>[2x]RLTSKQTFASFQQWAEKAEALGRDTEIGIYMIYKRDTPDTTPMNAAEQEHYLETLQALDNKKNLIIRPQIHDDREEEELDLGRYIAEDRNARTGFFRMVPKDQRAPETNSGRLTIGVEPKYGAQLALAMATLMDKHKSVTQGKVV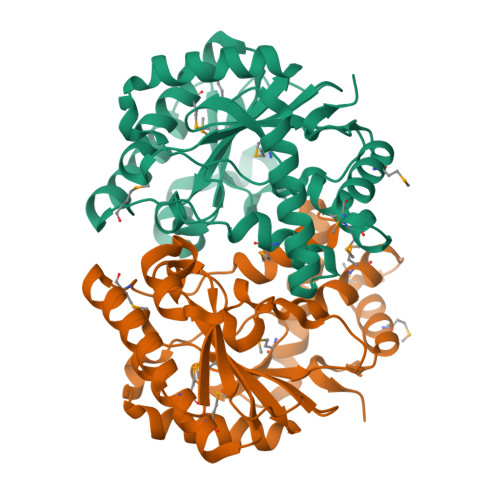GPAKYGQQTDSAILYINGDLAKAVKLGEKLKKLSGIPPEGFVEHTPLSMQSTGLGLSYAESVEGQPSSHGQARTHVIMDALKGQGPMENRLKMALAERGYDPENPALRAR> NLYFQGMRFVNPIPFVRDINRSKSFYRDRLGLKILEDFGSFVLFETGFAIHEGRSLEETIWRTSSDAQEAYGRRNMLLYFEHADVDAAFQDIAPHVELIHPLERQAWGQRVFRFYDPDGHAIEVGESLSQSGENLYFQGG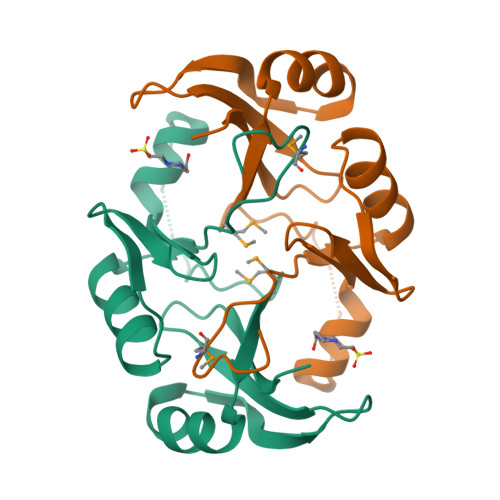S Even though constrained helical interaction motifs generally show a tendency to inhibit PPIs,1a only very few have been reported to directly target transcription factors with sufficient affinity to enable the inhibition of complex assembly.12a, 14 The nuclear transcription factor Y (NF‐Y)15 is a trimeric complex (NF‐YA/B/C) that binds to a particular DNA sequence (CCAAT box), thereby activating genes involved in regulation of the cell cycle and DNA repair. NF‐Y subunits B and C form a stable heterodimer, which by itself does not possess relevant affinity to DNA target sequences (CCAAT box DNA). Only upon availability and binding of the third subunit (NF‐YA) is the transcriptionally active trimeric complex formed and DNA binding occurs with affinity values in the low nanomolar range. In this study, we aimed to inhibit the interaction between the NF‐YB/C heterodimer (light/dark grey) and NF‐YA (green) to prevent transcription‐factor assembly and DNA (blue) binding.

Two derivatives of 19‐mer peptide 2‐D were synthesized, one lacking α‐methylation at position 272 (2‐DN, N‐terminal X) and the other at position 276 (2‐DC, C‐terminal X). Knowing that amino acid α‐methylation can restrict the conformational freedom of the peptide backbone, we investigated how variation of the α‐methyl pattern influences binding affinity of 2‐D. Only at position 272 did substitution of the methyl group by hydrogen affect binding, resulting in a peptide (2‐DN) with 15‐fold higher affinity. The highest affinity peptide 2‐DN was co‐crystalized with NF‐YB/C, yielding crystals diffracting up to 2.5 Å (space group P212121). For the higher‐affinity peptide (2‐DN), we obtained X‐ray and NMR structures in the NF‐YB/C‐bound form clearly showing contacts of the α‐helix and the extended N‐terminal stretch with the protein. The overlay of 2‐DN, 2‐C, and PBM in their bound state indicates an almost identical peptide conformation. When superimposed with its crystal structure (orange) in complex with NF‐YB/C, the NMR‐based conformers of bound 2‐DN (light orange) show a very good overlay. Notably, 2‐DN binding provides a thermodynamic profile similar to linear peptide 2, and it shows the highest entropic penalty (−TΔS=16.1 kcal mol−1) as well as the largest binding enthalpy (ΔH=−24.8 kcal mol−1) in our panel. Therefore, we reason that specific release of conformational constraint by removal of the α‐methyl group allows adaption of the correct binding mode. In the presence of peptide 2‐DN (c=10 μm), we observe a considerable loss in the fraction of bound DNA (32 % bound DNA).

> XVNAKQXHRIXKRRQARAKLX;> GPSFREQDIYLPIANVARIMKNAIPQTGKIAKDAKECVQECVSEFISFITSEASERCHQEKRKTINGEDILFAMSTLGFDSYVEPLKLYLQKFRE;> GPMEEIRNLTVKDFRVQELPLARIKKIMKLDEDVKMISAEAPVLFAKAAQIFITELTLRAWIHTEDNKRRTLQRNDIAMAITKFDQFDFLIDIVPR> IVGGENAKPGQFPWQVLLNGKIDAFCGGSIINEKWVVTAAHCIEPGVKITVVAGEYNTEETEPTEQRRNVIRAIPHHSYNATVNKYSHDIALLELDEPLTLNSYVTPICIADKEYTNIFLKFGSGYVSGWGRVFNRGRSATILQYLKVPLVDRATCLRSTKFTIYSNMFCAGFHEGGKDSCQGDSGGPHVTEVEGTSFLTGIISWGEECAVKGKYGIYTKVSRYVNWIKEKTKLT;> YNSGKLEEFVRGNLERECIEEKCSFEE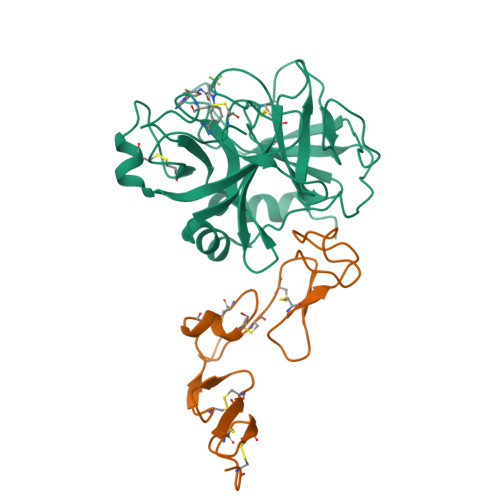AREVFENTEKTNEFWKQYVDGDQCEPNPCLNGGLCKDDINSYECWCQVGFEGKNCELDATCNIKNGRCKQFCKTGADSKVLCSCTTGYRLAPDQKSCKPAVPFPCGRVSVSHSPTTLTR>MSLVEATLEVIGGKWKCVILCHLTHGKKRTSELKRLMPNITQKMLTQQLRELEADGVINRIVYNQV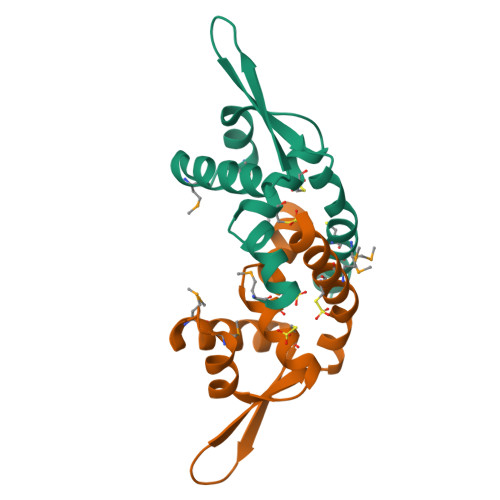PPKVEYELSEYGRSLEGILDMLCAWGANHINRVEGHHHHHH[4x]Starch phosphorylase (EC 2.4.1.1, α-d-glucosyl transferase; SP) catalyzes the reversible conversion of starch and inorganic phosphate into glucose-1-phosphate (Glc-1-P), playing an important role in starch metabolism in plants. S. tuberosum phosphorylase is the first starch phosphorylase discovered3−5 and has served as a model SP for biochemical studies of plant phosphorylases. The most significant structural difference between the Pho1 and Pho2 forms is a 78-residue-long peptide insertion in the middle of Pho1, termed the L78 segment. The stPho1ΔL78 structure reveals that activation of the enzyme occurs through the proteolytic degradation of the L78 segment and the association of the two remaining protein segments to form the active enzyme.

The free structure was solved from two different crystal forms that belonged in space groups P3121 and C2. In P3121, there is one stPho1ΔL78 molecule in the asymmetric unit, whereas in C2, there are three. stPho1ΔL78 structures from the two different crystal forms are almost identical, and since the structure from the crystal that belonged to P3121 was resolved at higher resolution (2.2 Å), we focused our analysis to this structure. stPho1 is composed by 916 residues.

>[3x]TLSEKIHHPITEQGGESDLSSFAPDAASITSSIKYHAEFTPVFSPERFELPKAFFATAQSVRDSLLINWNATYDIYEKLNMKQAYYLSMEFLQGRALLNAIGNLELTGAFAEALKNLGHNLENVASQEPDAALGNGGLGRLASCFLDSLATLNYPAWGYGLRYKYGLFKQRITKDGQEEVAEDWLEIGSPWEVVRNDVSYPIKFYGKVSTGSDGKRYWIGGEDIKAVAYDVPIPGYKTRTTISLRLWSTQVPSADFDLSAFNAGEHTKACEAQANAEKICYILYPGDESEEGKILRLKQQYTLCSASLQDIISRFERRSGDRIKWEEFPEKVAVQMNDTHPTLCIPELMRILIDLKGLNWNEAWNITQRTVAYTNHTVLPEALEKWSYELMQKLLPRHVEIIEAIDEELVHEIVLKYGSMDLNKLEEKLTTMRILENFDLPSSVAELFIKPEISVDDDTETVEVHDKVEASDKVVTNDEDDTGKKTSVKIEAAAEKDIDKKTPVSPEPAVIPPKKVRMANLCVVGGHAVNGVAEIHSEIVKEEVFNDFYELWPEKFQNKTNGVTPRRWIRFCNPPLSAIITKWTGTEDWVLKTEKLAELQKFADNEDLQNEWREAKRSNKIKVVSFLKEKTGYSVVPDAMFDIQVKRIHEYKRQLLNIFGIVYRYKKMKEMTAAERKTNFVPRVCIFGGKAFATYVQAKRIVKFITDVGATINHDPEIGDLLKVVFVPDYNVSVAELLIPASDLSEHISTAGMEASGTSNMKFAMNGCIQIGTLDGANVEIREEVGEENFFLFGAQAHEIAGLRKERADGKFVPDERFEEVKEFVRSGAFGSYNYDDLIGSLEGNEGFGRADYFLVGKDFPSYIECQEKVDEAYRDQKRWTTMSILNTAGSYKFSSDRTIHEYAKDIWNIEAVEIA> GVENSGAGPTSFKTMK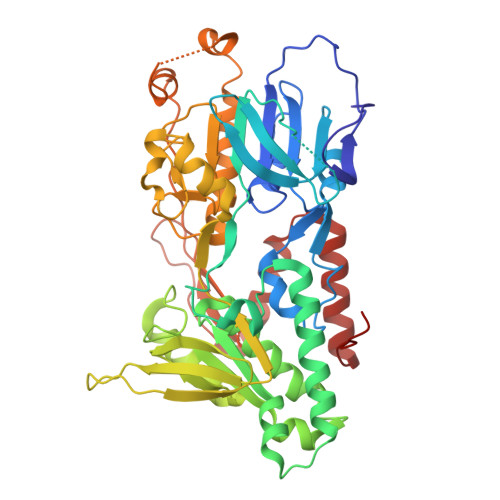VIDPQHSDKPNVLILGSGWGAISFLKHIDTKKYNVSIISPRSYFLFTPLLPSAPVGTVDEKSIIEPIVNFALKKKGNVTYYEAEATSINPDRNTVTIKSLSAVSQLYQPENHLGLHQAEPAEIKYDYLISAVGAEPNTFGIPGVTDYGHFLKEIPNSLEIRRTFAANLEKANLLPKGDPERRRLLSIVVVGGGPTGVEAAGELQDYVHQDLRKFLPALAEEVQIHLVEALPIVLNMFEKKLSSYAQSHLENTSIKVHLRTAVAKVEEKQLLAKTKHEDGKITEETIPYGTLIWATGNKARPVITDLFKKIPEQNSSKRGLAVNDFLQVKGSNNIFAIGDNAFAGLPPTAQVAHQEAEYLAKNFDKMAQIPNFQKNLSSRKDKIDLLFEENNFKPFKYNDLGALAYLGSERAIATIRSGKRTFYTGGGLMTFYLWRILYLSMILSARSRLKVFFDWIKLAFFKRDFFKGL(1,4-phenylene)bis(methylene) 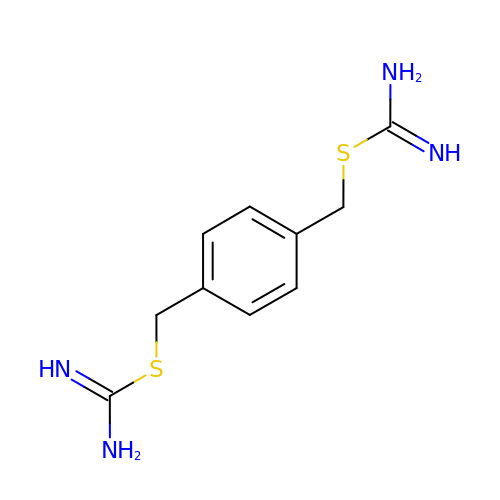dicarbamimidothioate | C10 H14 N4 S2 | PWMGHDCLHPWGBX-UHFFFAOYSA-N> MMPVFHTRTIESILEPVA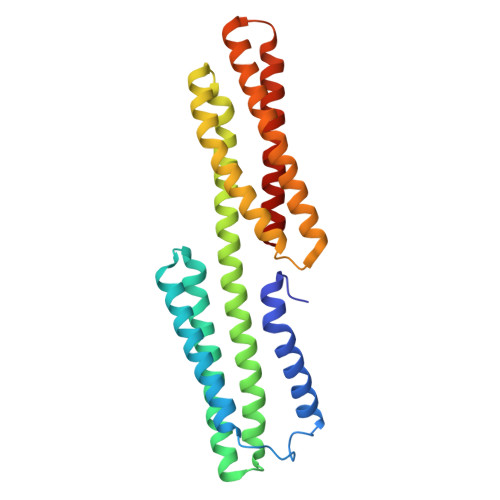QQISHLVIMHEEGEVDGKAIPDLTAPVAAVQAAVSNLVRVGKETVQTTEDQILKRDMPPAFIKVENACTKLVQAAQMLQSDPYSVPARDYLIDGSRGILSGTSDLLLTFDEAEVRKIIRVCKGILEYLTVAEVVETMEDLVTYTKNLGPGMTKMAKMIDERQQELTHQEHRVMLVNSMNTVKELLPVLISAMKIFVTTKNSKNQGIEEALKNRNFTVEKMSAEINEIIRVLQLTS>[4x]AFELPSLPYAIDALEPHISKETLEFHHGKHHNTYVVKLNGLIPGTKFENKSLEEIVCSSDG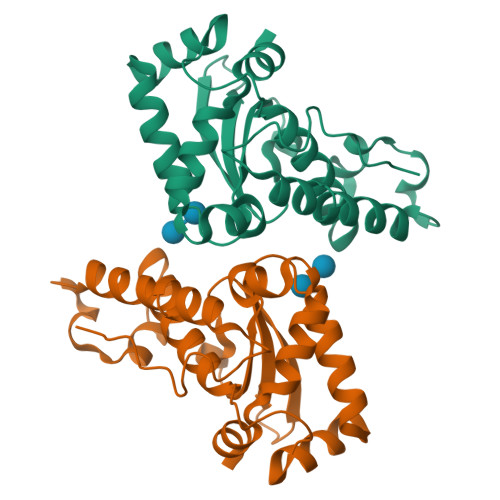GVFNNAAQIWNHTFYWNSLSPNGGGAPTGAVADAINAKWGSFDAFKEALNDKAVNNFGSSWTWLVKLADGSLDIVNTSNAATPLTDDGVTPILTVDLWEHAYYIDYRNVRPDYLKGFWSLVNWEFANANFA>MGKVYVFDHPLIQHKLTYIRDKNTGTKEFRELVDEVATLMAFEITRDLPLEEVEIETPVSKARAKVIAGKKLGVIPILRAGIGMVDGILKLIPAAKVGHIGLYRDPQTLKPVEYYVKLPSDVEERDFIIVDPMLATGGSAVAAIDALKKRGAKSIKFMCLIAAPEGVKAVETAHPDV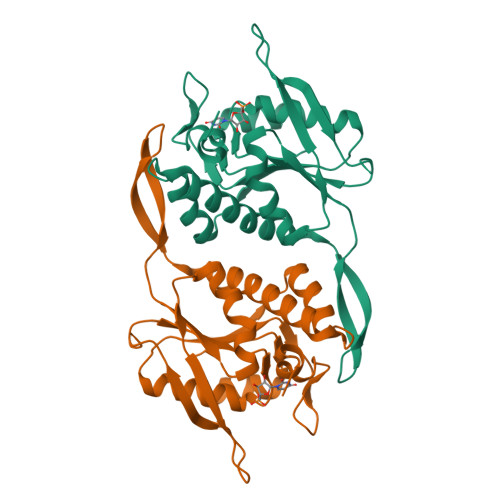DIYIAALDERLNDHGYIVPGLGDAGDRLFGTK[2x]Shiga toxin (Stx), a major virulence factor of enterohemorrhagic Escherichia coli (EHEC), can cause fatal systemic complications. All Stx proteins consist of a catalytic A-subunit and a B-subunit pentamer. The catalytic A-subunit, which is a member of ribosome-inactivating proteins (RIPs), has an RNA N-glycosidase activity that cleaves a specific adenine from 28S ribosomal RNA to inhibit eukaryotic protein synthesis. The B-subunit pentamer functions to bind Galα[1–4]–Galβ[1–4]–Glcβ-ceramide (Gb3), a glycolipid present on the surface of target cells.

To elucidate the precise manner by which these shorter peptides bind to Stx2a, X-ray crystallography analysis was performed with co-crystals of each peptide and the Stx2a holotoxin, which were obtained via the soaking method. We were able to determine electron densities for AR4A-mono, R4A-mono, R3A-mono, and R2A-mono, and X-ray crystal structures were solved to final resolutions of 1.80, 1.80, 1.90, and 1.75 Å-resolution, respectively. These structures reveal that the AR4A-mono, R4A-mono, R3A-mono, and R2A-mono peptides bind tightly to the catalytic A-subunit. In all cases, the common Arg8-Arg9-Ala10 motif (numbering reflects residue position in full-length MMβA-mono) interacts equally with the Glu72, Tyr77, Val78, Asp94, Ser112, Tyr114, Thr115, Glu167, Arg170, Thr199, and Gly203 residues present in the catalytic pocket of the A-subunit, whereas the Arg8 and Arg9 residues of the motif electrostatically interact with Glu167 and Asp94, respectively. The amide group of the Ala10, but not its side chain, interacts with the Val78, Ser112 and Arg170 residues. In addition, Arg6 and Arg7 of both AR4A-mono and R4A-mono electrostatically interact, respectively, with Asp94 of the A-subunit and Asp70 of the B-subunit, which is adjacent to the catalytic cavity. Overall, we find that the binding patterns of these shorter peptides are almost identical to that of MMβA-mono. We found that R4-mono, AR4A-mono, R4A-mono, and R3-mono exhibit greater inhibitory effects (relative IC50 values = 0.387, 2.27, 2.70, and 3.68 µM, respectively) than non-tagged MMβA-mono (relative IC50 = 8.14 µM), which was used as a positive control to compete the binding. Although the precise mechanism of the detrimental effect of the C-terminal Ala is remained to be elucidated, the presence of the amide group of the C-terminal Ala may contribute to fix the binding manner of the peptides with this Ala, such as MMbA-mono, AR4A-mono, R4A-mono, R3A-mono, and R2A-mono, to the same orientations which are clearly demonstrated in their crystal structures.

> REFTIDFSTQQSYVSSLNSIRTEISTPLEHISQGTTSVSVINHTPPGSYFAVDIRGLDVYQARFDHLRLIIEQNNLYVAGFVNTATNTFYRFSDFTHISVPGVTTVSMTTDSSYTTLQRVAALERSGMQISRHSLVSSYLALMEFSGNTMTRDASRAVLRFVTVTAEALRFRQIQREFRQALSETAPVYTMTPGDVDLTLNWGRISNVLPEYRGEDGVRVGRISFNNISAILGTVAVILNCHHQGARSVRAVNEESQPECQITGDRPVIKINNTLWESNTAAAFLNRKSQFLYTTGK;>ADCAKGKIEFSKYNEDDTFTVKVDGKEYWTSRWNLQPLLQSAQLTGMTVTIKSSTCESGSGFAEVQFNND[5x];> ARRRRAX(3R)-oct-1-en-3-ol | C8 H16 O | 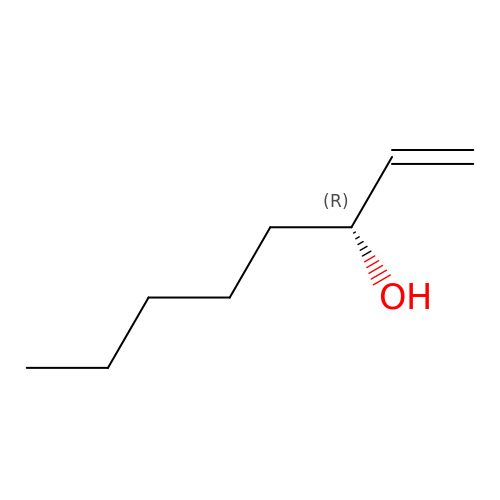VSMOENVRRABVKN-QMMMGPOBSA-N>[2x]MDLTVEPNLHSLITSTTHKWIFVGGKGGVGKTTSSCSIAIQMALSQPNKQFLLISTDPAHNLSDAFGEKFGKDARKVTGMNNLSCMEIDPSAALKDM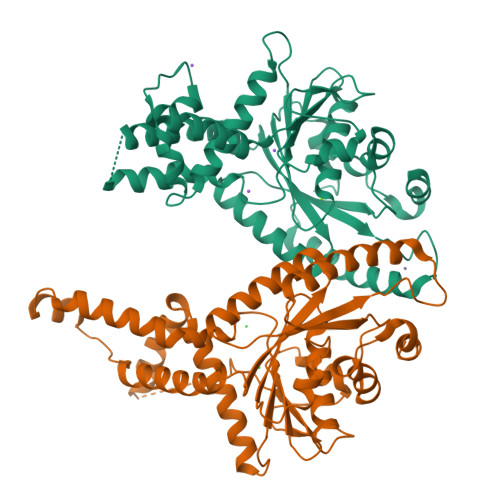NDMAVSRANNNGSDGQGDDLGSLLQGGALADLTGSIPGIDEALSFMEVMKHIKRQEQGEGETFDTVIFDTAPTGHTLRFLQLPNTLSKLLEKFGEITNKLGPMLNSFMGAGNVDISGKLNELKANVETIRQQFTDPDLTTFVCVCISEFLSLYETERLIQELISYDMDVNSIIVNQLLFAENDQEHNCKRCQARWKMQKKYLDQIDELYEDFHVVKMPLCAGEIRGLNNLTKFSQFLNKEYNPITDGKVIYELEDKE>[2x]GSEFTQLSQSIAEFHTYQLGNGRCSSLLAQRIHAPPETVWSVVRRFDR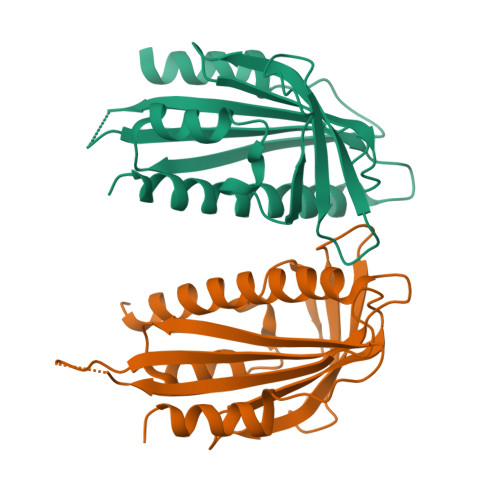PQIYKHFIKSCNVSEDFEMRVGCTRDVNVISGLPANTSRERLDLLDDDRRVTGFSITGGEHRLRNYKSVTTVHRFEKEEEEERIWTVVLESYVVDVPEGNSEEDTRLFADTVIRLNLQKLASITEAMNRN isoquercetin | C21 H20 O12 | 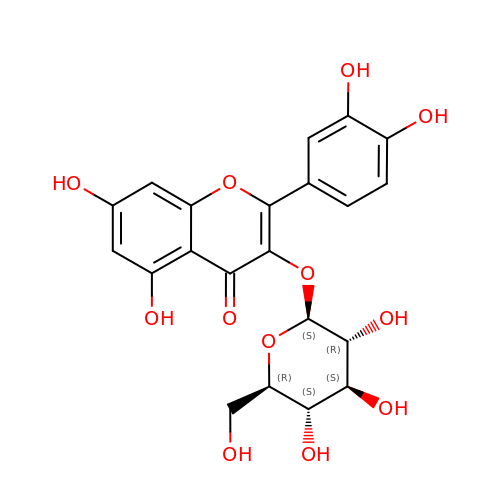OVSQVDMCBVZWGM-QSOFNFLRSA-N> GMTDWQQALDRHVGVGVRTTRDLIRLIQPEDWDKRPISGKR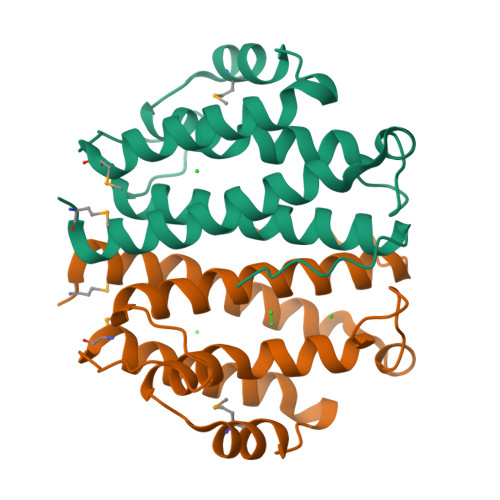SVYEVAVHLAVLLEADLRIATGATADEMAQFYAVPVLPEQLVDRLDQSWQYYQDRLMADFSTETTYWGVTDSTTGWLLEAAVHLYHHRSQLLDYLNLLGYDIKLDLFE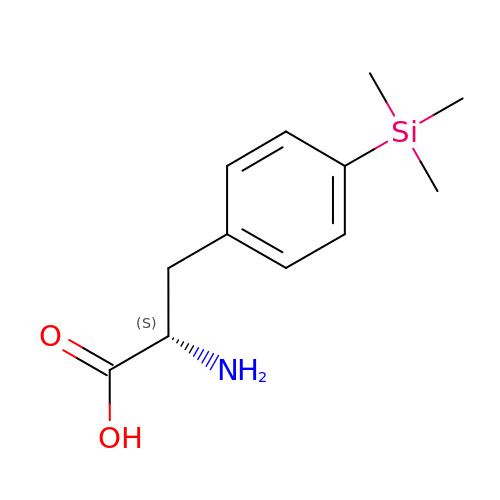4-(trimethylsilyl)-L-phenylalanine | C12 H19 N O2 Si | YJYWOZDNAZTLQC-NSHDSACASA-N>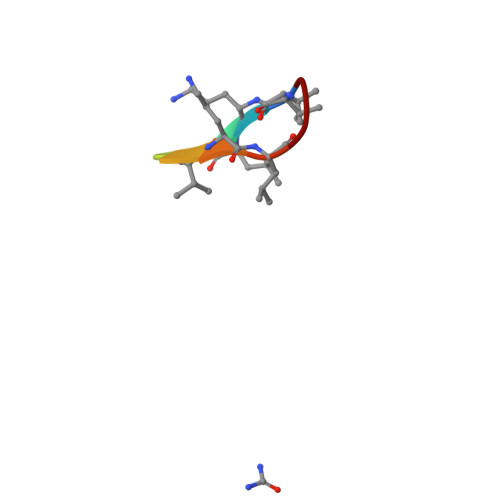 VALFPVALFP>MPPETATNPKDARHDGWQTLKRFLPYLWPADNAVLRRRVVGAILMVLLGKATTLALPFAYKKAVDAMTLGGGAQPALTVALAFVLAYALGRFSGVLFDNLRNIVFERVGQDATRHLAENVFARLHKLSLRFHLARRTGEVTKVIERGTKSIDTMLYFLLFNIAPTVIELTAVIVIFWLNFGLGLVTATILAVIAYVWTTRTITEWRTHLREKMNRLDGQALARAVDSLLNYETVKYFGAESREEARYASAARAYADAAVKSENSLGLLNIAQALIVNLLMAGAMAWTVYGWSQGKLTVGDLVFVNTYLTQLFRPLDMLGMVYRTIRQGLIDMAEMFRLIDTHIEVADVPNAPALVVNRPSVTFDNVVFGYDRDREILHGLSFEVAAGSRVAIVGPSGAGKSTIARLLFRFYDPWEGRILIDGQDIAHVTQTSLRAALGIVPQDSVLFNDTIGYNIAYGRDGASRAEVDAAAKGAAIADFIARLPQGYDTEVGERGLKLSGGEKQRVAIARTLVKNPPILLFDEATSALDTRTE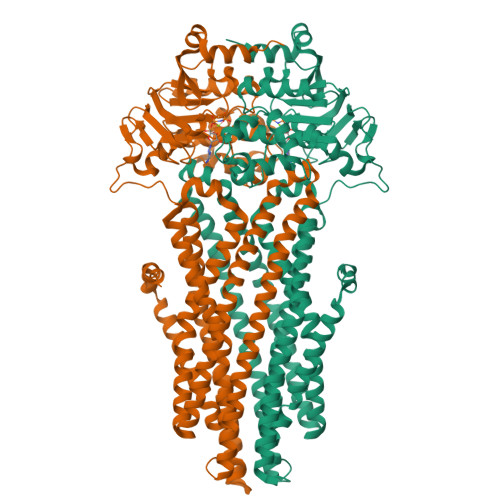QDILSTMRAVASHRTTISIAHRLSTIADSDTILVLDQGRLAEQGSHLDLLRRDGLYAEMWARQAAESAEVSEAAEHHHHHH[6x]> GSSHHHHHHSSGLVPRGSHMGSIIDAAAAAGPVVLMETAFRKAVESRQIPGAVIMARDASGNLNYTRCFGARTVRRDENNQLPPLQVDTPCRLAAATKLLTTIMVLQCMERGLVDLDETVDRLLPDLSAMPVLEGFDDAGNARLRERRGKITLRHLLTHTSGLSYVFLHPLLREYMAQGYLQSAEKFGIQSRLAPPAVNDPGAEWIYGTNLDWAGKLVERATGLDLEQYLQENICAPLGIT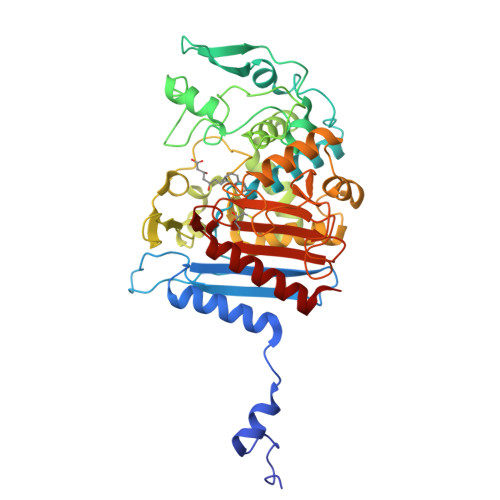DMTFKLQQRPDMLARRADQTHRNSADGRLRYDDSVYFRADGEECFGGQGVFSSPGSYMKVLHSLLKRDGLLLQPQTVDLMFQPALEPRLEEQMNQHMDASPHINYGGPMPMVLRRSFGLGGIIALEDLDGENWRRKGSLTFGGGPNIVWQIDPKAGLCTLAFFQLEPWNDPVCRDLTRTFEHAIYAQYQQG>GSHMMPGEIRPTIGQQMETGDQRFGDLVFRQLAPNVWQHTSYLDMPGFGAVASNGLIVRDGGRVLVVDTAWTDDQTAQILNWIKQEINLPVALAVVTHAHQDKMGGMDALHAAGIATYANALSNQLAPQEGMV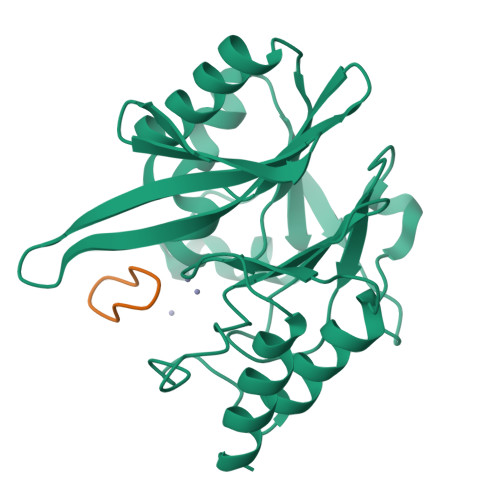AAQHSLTFAANGWVEPATAPNFGPLKVFYPGPGHTSDNITVGIDGTDIAFGGCLIKDSKAKSLGNLGDADTEHYAASARAFGAAFPKASMIVMSHSAPDSRAAITHTARMADKLR[4x];>[4x]RRLCPIPE>[2x]HHHHHHMKILFLDQSGKPGGAELCLIDIAKPYRDRALVGLFADGAFKTLLEQHHIPVEVFTNQPIQVRKQSNLLQAFGSLGQLAPLVAKVVQTAHEYDLIYANTQKALVVGAIASFIARRPLVYHLHDILSPEHFSQTNLRVAVNLANRFASLVIANSQASQTAFIQAGGRAELTKVIYNGFDINLYKTSPSDISKLRQQLGVANNFVVG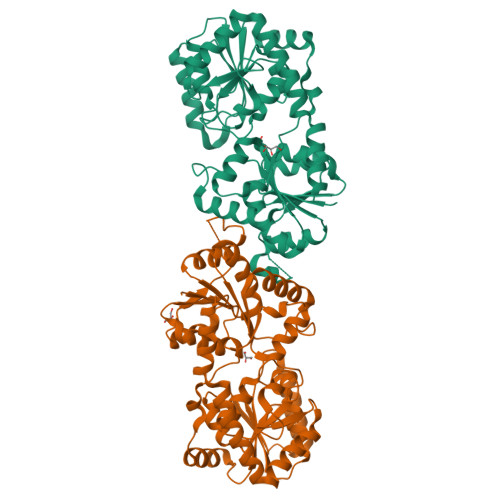HFSRLSPWKGQHILIDALAQCPPQVTAILVGDALFGEQDYVKELHQQITRLGLENRVKFLGFRADIPQLMAACDLVAHTSTAPEPFGRVIVEAMLCGKPVVAAKAGGAMELVEHGVNGFLTTPGESQELANIINTCIEDTQKTATIASNAQAIASQRFDVVTINQQIAETLSSLGFTR> SASPQEQDQDRRKDWGHVELLEVLQARVRQLQAESVSEVVVNRVDVARLPECGSGDGSLQPPRKVQMGAKDATPVPCGRWAKILEKDKRTQQMRMQRLKAKLQMPFQSGEFKALTRRLQVEPRLLSKQMAGCLEDCTRQAPESPWEEQLARLLQEAPGKLSLDVEQAPSGQHSQAQLSGQQQRLLAFFKCCLLTDQLPLAHHLLVVHHGQRQKRKLLTLDMYNAVMLGWARQGAFKELVYVLFMVKDAGLTPDLLSYAAALQCMGRQDQDAGTIERCLEQMSQEGLKLQALFTAVLLSEEDRATVLKAVHKVKPTFSLPPQLPPPVNTSKLLRDVYAKDGRVSYPKLHLPLKTLQCLFEKQLHMELASRVCVVSVEKPTLPSKEVKHARKTLKTLRDQWEKALCRALRETKNRLEREVYEGRFSLYPFLCLLDEREVVRMLLQVLQALPAQGESFTTLARELSARTFSRHVVQRQRVSGQVQALQNHYRKYLCLLASDAEVPEPCLPRQYWEELGAPEALREQPWPLPVQMELGKLLAEMLVQATQMPCSLDKPHRSSRLVPVLYHVYSFRNVQQIGILKPHPAYVQLLEKAAEPTLTFEAVDVPMLCPPLPWTSPHSGAFLLSPTKLMRTVEGATQHQELLETCPPTALHGALDALTQLGNCAWRVNGRVLDLVLQLFQAKGCPQLGVPAPPSEAPQPPEAHLPHSAAPARKAELRRELAHCQKVAREMHSLRAEALYRLSLAQHLRDRVFWLPHNMDFRGRTYPCPPHFNHLGSDVARALLEFAQGRPLGPHGLDWLKIHLVNLTGLKKREPLRKRLAFAEEVMDDILDSADQPLTGRKWWMGAEEPWQTLACCMEVANAVRASDPAAYVSHLPVHQDGSCNGLQHYAALGRDSVGAASVNLEPSDVPQDVYSGVAAQVEVFRRQDAQRGMRVAQ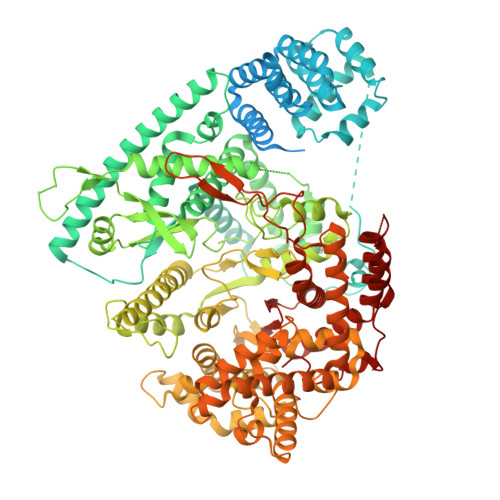VLEGFITRKVVKQTVMTVVYGVTRYGGRLQIEKRLRELSDFPQEFVWEASHYLVRQVFKSLQEMFSGTRAIQHWLTESARLISHMGSVVEWVTPLGVPVIQPYRLDSKVKQIGGGIQSITYTHNGDISRKPNTRKQKNGFPPNFIHSLDSSHMMLTALHCYRKGLTFVSVHDCYWTHAADVSVMNQVCREQFVRLHSEPILQDLSRFLVKRFCSEPQKILEASQLKETLQAVPKPGAFDLEQVKRSTYFFS>MDFSRNLYDIGEQLDSEDLASLKFLSLDYIPQRKQEPIKDALMLFQRLQEKRMLEESNLSFLKELLFRINRLDLLITYLNTRKEEMERELQTPGRAQISAYRVMLYQISEEVSRSELRSFKGGLQEEISKCKLDDDMNLLDIFIEMEKRVILGEGKLDILKRVCAQINKSLLKIINDYEEFSKER[4x];>GSHMSAEVIGQVEEALDTDEKEMLLFLCRDVAIDVVPPNVRDLLDILRERGKLSVGDLAELLYRVRRFDLLKRILKMDRKAVETHLLRNPHLVSDYRVLMAEIGEDLDKSDVSSLIFLMKDYMGRGKISKEKSFLDLVVELEKLNLVAPDQLDLLEKCLKNIH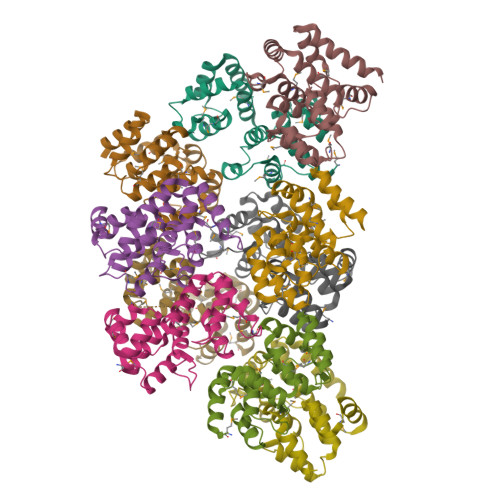RIDLKTKIQKYKQSVQGAGTS[6x]>MSYSGERDNFAPHMALVPMVIEQTSRGERSFDIYSRLLKERVIFLTGQVEDHMANLIVAQMLFLEAENPEKDIYLYINSPGGVITAGMSIYDTMQFIKPDVSTICMGQAASMGAFLLTAGAKGKRFCLPNSRVMIHQPLGGYQGQATDIEIHAREIL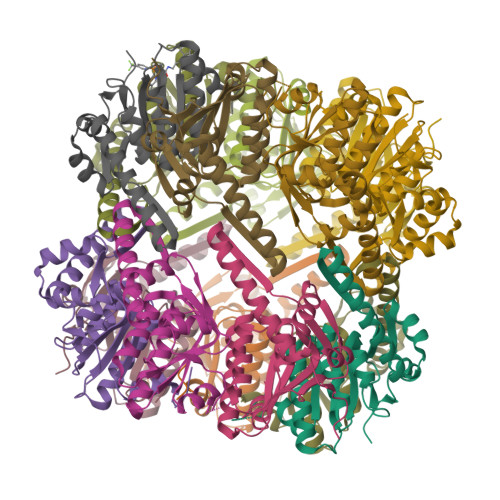KVKGRMNELMALHTGQSLEQIERDTERDRFLSAPEAVEYGLVDSILTHRN[28x]>[2x]KNTSAPSQQEPDRFDRDRLFSVVSRGVPEELTGLLEYLRWNSKYLTDSAYTEGSTGKTCLMKAVLNLQDGVNACIMPLLQIDKDSGNPKPLVNAQCTDEFYQGHSALHIAIEKRSLQCVKLLVENGADVHLRACGRFFQKHQGTCFYFGELPLSLAA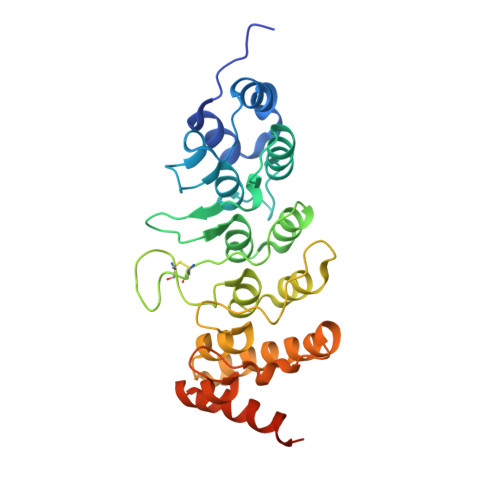CTKQWDVVTYLLENPHQPASLEATDSLGNTVLHALVMIADNSPENSALVIHMYDGLLQMGARLCPTVQLEEISNHQGLTPLKLAAKEGKIEIFRHILQREFSGPYQPLAAAHHHHHH PHOSPHORIC ACID MONO-(2,3,4,6-TETRAHYDROXY-5-PHOSPHONOOXY-CYCLOHEXYL) ESTER | C6 H14 O12 P2 | 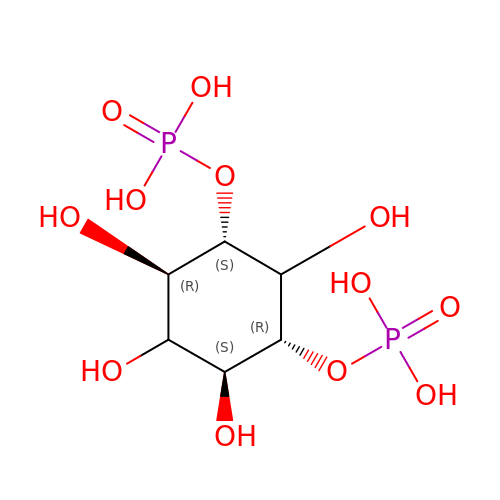PUVHMWJJTITUGO-FICORBCRSA-N>[2x]GPAGAQDDVPPYFKTEPVRTQVHLEGNRLVLTCMAEGSWPLEFKWLHNNRELTRFSLEYRYMITSLDRTHAGFYRCIVRNRMGALLQRQTEVQVAYMGSFEEGEKRQSVNHGEAAVIRAPRISSFPRPQVTWFRDGRKIPPSSRIAITLENTLVILSTVAPDAGRYYVQAVNDKNGDNKTSQPITLAVENVGGPADPIAPTIIIPPKNTSVVAGT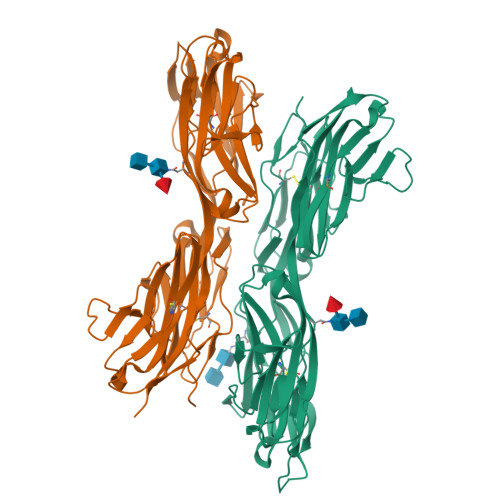SEVTMECVANARPLIKLHIVWKKDGAPLSSGISDYNRRLTIANPTVSDAGYYECEAMLRSSSVAPVTRGAYLSVLEPPQFVREPERHITAEMEKVVDIPCRAKGVPPPSITWYKDAALVEVGKLTRFKQRSDGGLQISGLLPDDTGMLQCFAHNAAGEAQTSTYLAVTS> MLEQPYLDLAKKVLDEGHFKPDRTHTGTYSIFGHQMRFDLSKGFPLLTTKKVPFGLIKSELLWFLHGDTNIRFLLQHRNHIWDEWAFEKWVKSDEYHGPDMTDFGHRSQKDPEFAAVYHEEMAKFDDRVLHDDAFAAKYGDLGLVYGSQWRAWHTSKGDTIDQLGDVIEQIKTHPYSRRLIVSAWNPEDVPTMALPPCHTLYQFYVNDGKLSLQLYQRSADIFLGVPFCIASYALLTHLVAHECGLEVGEFIHTFGDAHLYVNHLD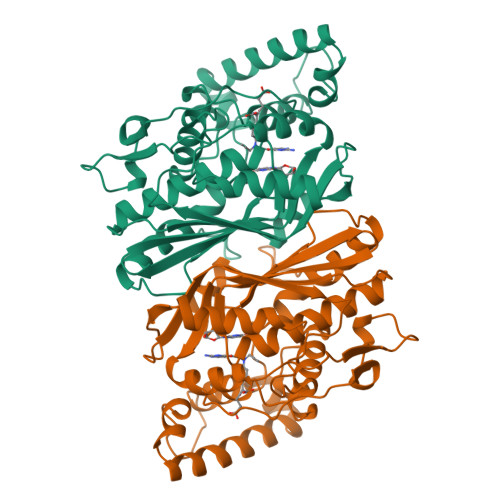QIKEQLSRTPRPAPTLQLNPDKHDIFDFDMKDIKLLNYDPYPAIKAPVAV> MAFAKELFLGKIKKKEVFPFPEVSQDELNEINQFLGPVEKFFTEEVDSRKIDQEGKIPDETLEKLKSLGLFGLQVPEEYGGLGFSNTMYSRL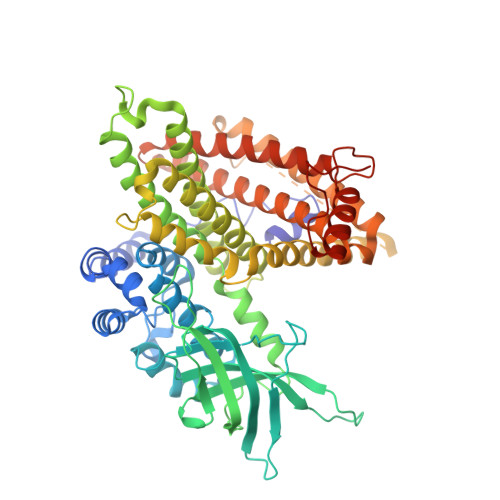GEIISMDGSITVTLAAHQAIGLKGIILAGTEEQKAKYLPKLASGEHIAAFCLTEPASGSDAASIRSRATLSEDKKHYILNGSKVWITNGGLANIFTVFAKTEVVDSDGSVKDKITAFIVERDFGGVTNGKPEDKLGIRGSNTCEVHFENTKIPVENILGEVGDGFKVAMNILNSGRFSMGSVVAGLLKRLIEMTAEYACTRKQFNKRLSEFGLIQEKFALMAQKAYVMESMTYLTAGMLDQPGFPDCSIEAAMVKVFSSEAAWQCVSEALQILGGLGYTRDYPYERILRDTRILLIFEGTNEILRMYIALTGLQHAGRILTTRIHELKQAKVSTVMDTVGRRLRDSLGRTVDLGLTGNHGVVHPSLADSANKFEENTYCFGRTVETLLLRFGKTIMEEQLVLKRVANILINLYGMTAVLSRASRSIRIGLRNHDHEVLLANTFCVEAYLQNLFSLSQLDKYAPENLDEQIKKVSQQILEKRAYICAHPLDRTCHHHHHH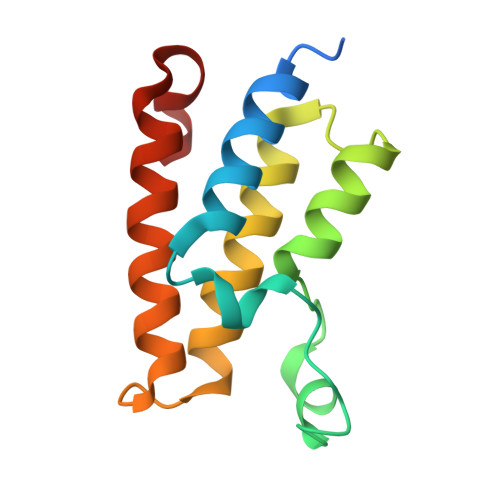> AMANIAQRPKRGPHDAAIQNILTELQNHAAAWPFLQPVNKEEVPDYYDFIKEPMDLSTMEIKLESNKYQKMEDFIYDARLVFNNCRMYNGENTSYYKYANRLEKFFNNKVKEIPEYSHLID> EQGNRPVETENIA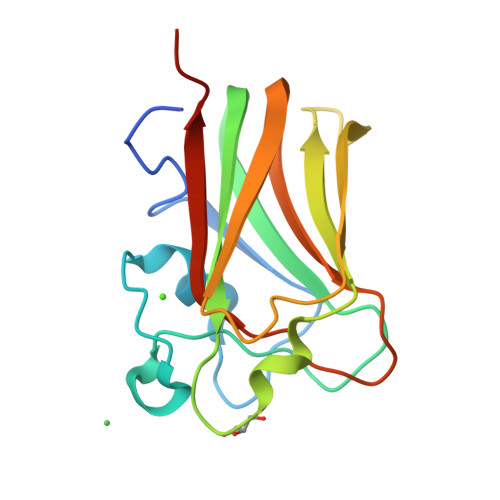RGKQASQSSTAYGGAATRAVDGNVDSDYGHHSVTHTNFEDNAWWQVDLGKTENVGKVKLYNRGDGNVANRLSNFDVVLLNEAKQEVARQHFDSLNGKAELEVFFTAKDARYVKVELKTKNTPLSLAEVEVFRSATTQVGC> GAMDPMKAKRVQAKIEMEFPSEDVAKVVYEAVLYEHLSVPYRRSEIDFKLEGKKIIL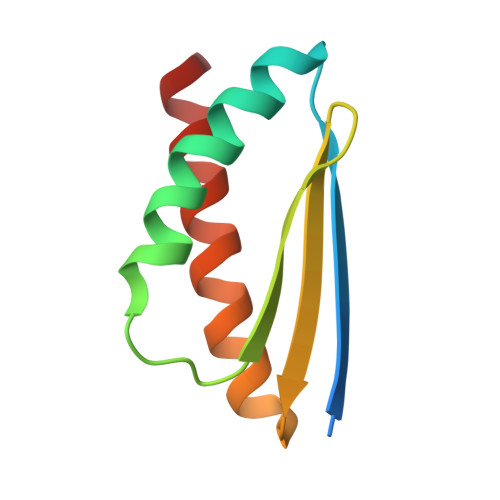DIKATDSSALRGTVNSYLRWIKAAIDVIEV>[2x]MGSSHHHHHHHHHHSSGLVPRGSHVAPPNLTREQAEQRAALLEVQSYAIELDLSAGAGGPEVETFGSTTTVRFRSATPGAESWIDLVAARVRSAVLNGVELDVSDYDESTGIRLPELAADNELVVHADCQYTNTGEGLHRFIDPVDGGVYLYSQFETADAKRMF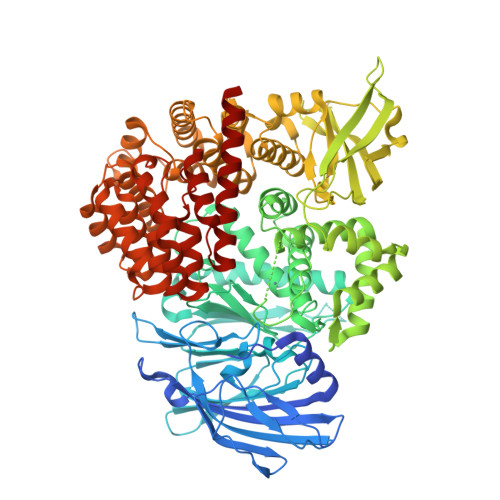TCFDQPDLKATYQITVTAPQDWKVISNAAGEVTDTGEGTRRHVFDTTKPMSTYLVALVAGPYAEWRDVFPGDDGQDEIPLGIYCRASLAEHLDAERLFIETKQGFGFFHKAFGVPYPFGKYDQCFVPEFNAGAMENAGCVTFLEDYVFRSRVTGYLYERRSETVLHEMAHMWFGDLVTMRWWDDLWLNESFATWASVLAQVGATQYTNAWTTFASVEKSWAYRQDQLPSTHPVAADIPDLQAVEVNFDGITYAKGASVLKQLVAYVGLENFLAGLKVYFDRHAWGNATLDDLLVALEEASGRDLSWWSAQWLQTTGLNMLRPKLAIDDEGRFTSFSVLQSPARPGAGEHRTHRLAIGIYDDDPATGELVRTHRVELDVTGERTEVPDLVGVHRGKLVLVNDDDLTYCTMRLDPQSLATLIDRIADIQESLPRALCWSTAWEMTREAELKARDFVSLVLGSSPTTGIGAESEIGVVQRVLLQTQTALASYADPAWQPEGWRRFAGRLLELARAAEPGSDHQLAFVNSLAGSVLGEEQISAMRGWLDGTAPLEGLTVDTDLRWGLLQALVAHGAAGEAEIDAELERDQTATGRRRAERARSLIPTPEAKEKAWQRAVHDDQLPNAISDAIISGFQHPGQRELLASYVRRYFDEIDEVWHRRSSERAQPTVIGLFPSWAVDEDTVAVADRWLEGEHAPALRRLVSEGRAGIVRALAAREFDRS>MAHHHHHHMVQRIAMAPQGPEFSRFVMGYWRLMDWKMSPGELVSFIEQHLDLGVTTVDHADIYGDYQCEAAFGEALKRAPHLRSRMEIVSKCGIATRARAENTIGHYITDRDHIVLSAEQSLRNLATDHLDLLLIHRPDPLMDADEVAEAFLALHHSGKVRHFGVSNFTPAQFTLLQSRLPFTLATNQVEISPVHQPLLLDGTLDQLQQLRIRPMAWSCLGGGRLFNEEC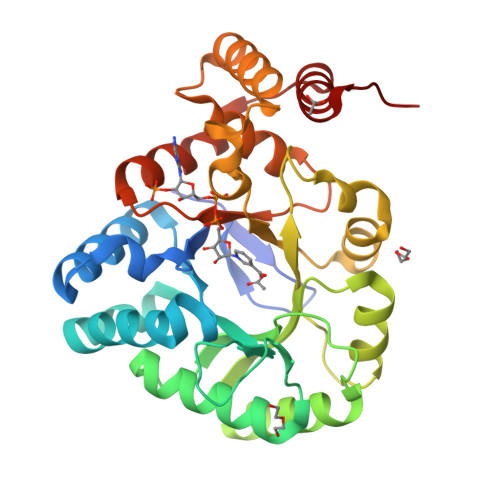FQALRDELAQVAHELNADSIEQVVYAWVLRLPSQPLPIIGSGKIERVRSAIVAEKLSMTRQQWFRIRKAALGYDVP[6x]> GTGCGTGTGACTGT;> ACGGACAGTCACACGC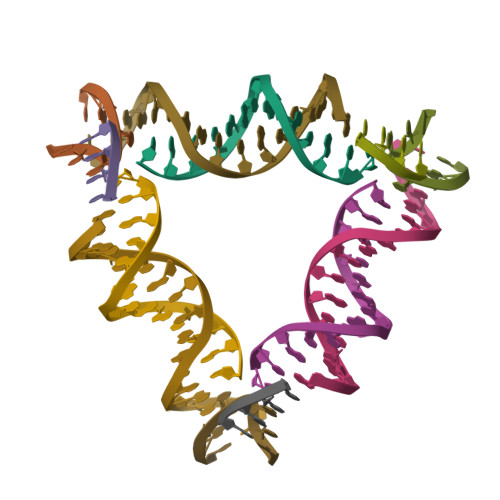A;> ACACCGT;> CTGTA> 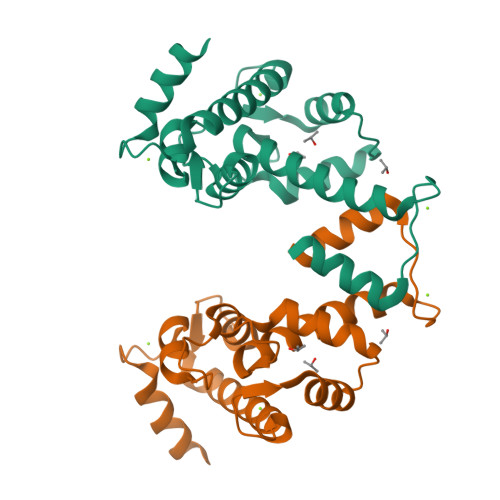MDQSFLWNVFQRVDKDRSGVISDNELQQALSNGTWTPFNPVTVRSIISMFDRENKAGVNFSEFTGVWKYITDWQNVFRTYDRDNSGMIDKNELKQALSGFGYRLSDQFHDILIRKFDRQGRGQIAFDDFIQGCIVLQRLTDIFRRYDTDQDGWIQVSYEQYLSMVFSIV>PNYKLTYFNMRGRAEIIRYIFAYLDIQYEDHRIEQADWPEIKSTLPFGKIPILEVDGLTLHQSLAIARYLTKNTDLAGNTEMEQCHVDAIVDTLDDFMSCFPWAEKKQDVKEQMFNELLTYNAPHLMQDLDTYLGGREWLIGNSVTWADFYWEICSTTL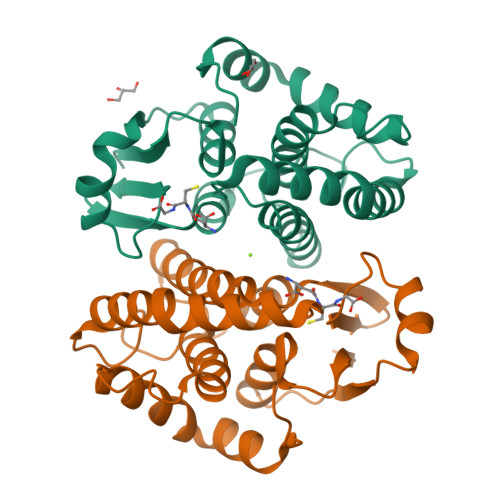LVFKPDLLDNHPRLVTLRKKVQAIPAVANWIKRRPQTKL[4x]> MSAILKRAAKYKRVSSILCEGEAHLRDPFTPPPVILKPPAPRKDKKPDDITDFPAQKLIPLPESIPYQEGKYRPASI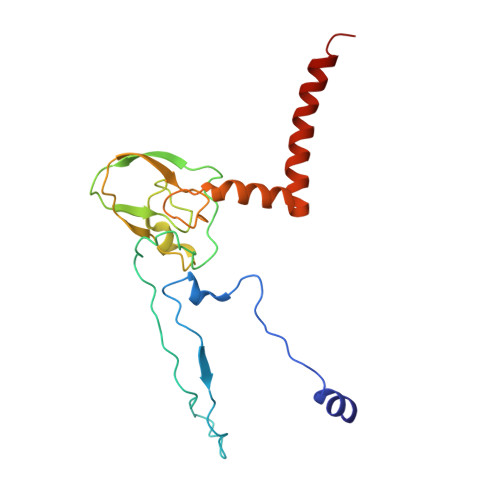PMVAGFFPYNCYLQQGKVYSWCSCGISQSGPWCDGLCNSVVTRCRPVVFNVSQSGYYKICNCKFSANAPFCNNTHRKMVRYHHQTHRGFYEIWGAALFVLGWVYMGFNYYT> AAGSTQAQAAPFPELCSYTWEAVDTKNNVLYKINICGSVDIVQCGPSSAVCMHDLKTRTYHSVGDSVLRSATRSLLEFNTTVSCDQQGTNHRVQSSIAFLCGKTLGTPEFVTATECVHYFEWRTTAACKKDIFKANKEVPCYVFDEELRKHDLNPLIKLSGAYLVDDSDPDTSLFINVCRDIDTLRDPGSQLRACPPGTAACLVRGHQAFDVGQPRDGLKLVRKDRLVLSYVREEAGKLDFCDGHSPAVTITFVCPSERREGTIPKLTAKSNCRYEIEWITEYACHRDYLESKTCSLSGEQQDVSIDLTPLAQSGGSSYISDGKEYLFYLNVCGETEIQFCNKKQAAVCQVKKSDTSQVKAAGRYHNQTLRYSDGDLTLIYFGGDECSSGFQRMSVINFECNKTAGNDGKGTPVFTGEVDCTYFFTWDTEYACVKEKEDLLCGATDGKKRYDLSALVRHAEPEQNWEAVDGSQTETEKKHFFINICHRVLQEGKARGCPEDAAVCAVDKNGSKNLGKFISSPMKEKGNIQL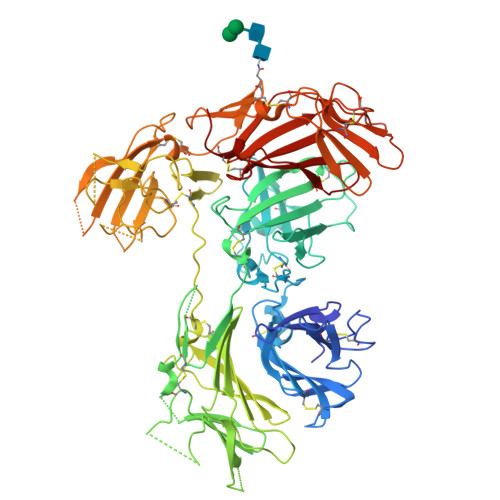SYSDGDDCGHGKKIKTNITLVCKPGDLESAPVLRTSGEGGCFYEFEWHTAAACVLSKTEGENCTVFDSQAGFSFDLSPLTKKNGAYKVETKKYDFYINVCGPVSVSPCQPDSGACQVAKSDEKTWNLGLSNAKLSYYDGMIQLNYRGGTPYNNERHTPRATLITFLCDRDAGVGFPEYQEEDNSTYNFRWYTSYACPEEALVPL> FNIVGTT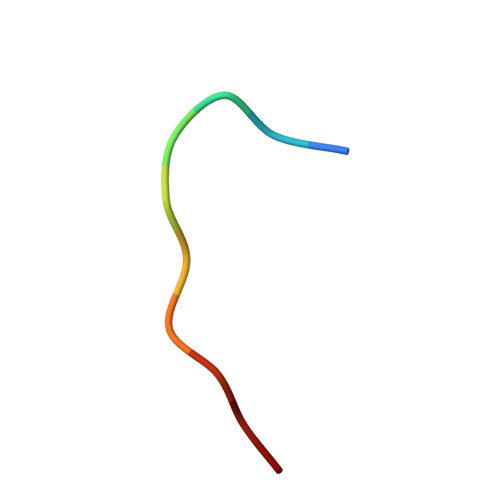YPC>MAKGGSRVSNPAVMAQ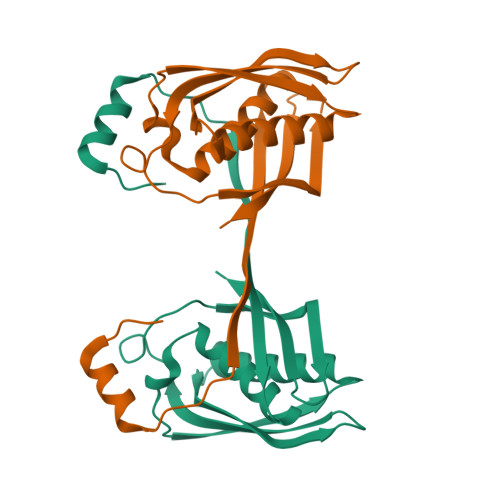EEEDVRDYNLTEEQKAIKAKYPPVNRKYEYLDHTAAVQLHAWGDTLEEAFEQCAMAMFGYMTDTGTVEPLQTVEVETQGDDLQSLLFHFLDEWLYKFSADEFFIPREVKVLSIDQRNFKLRSIGWGEEFSLSKHPQGTEVKAITYSAMQVYNEENPEVFVIIDILEHHHHHH[2x]>[2x]GHMENKVINFKKIIDSRGSLVAIE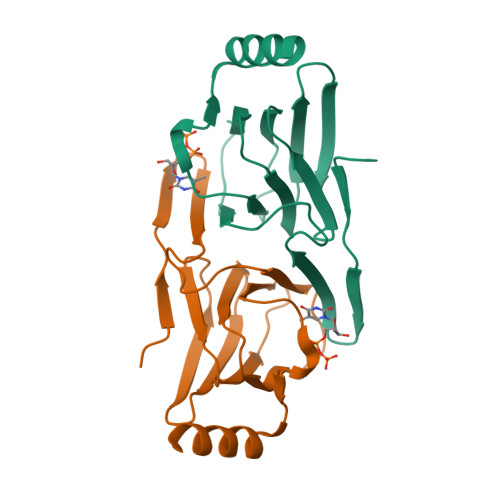ENKNIPFSIKRVYYIFDTKGEEPRGFNAHKKLEQVLVCLNGSCRVILDDGNIIQEITLDSPAVGLYVGPAVWHEMHDFSSDCVMMVLASDYYDETDYIRQYDNFKKYIAKINLEKEG> MSGVRAVRISIESACEKQVHEVGLDGTETYLPPLSMSQNLARLAQRIDFSQGSGSEEEEAAGTEGDAQEWPGAGSSADQDDEEGVVKFQPSLWPWDSVRNNLRSALTEMCVLYDVLSIVRDKKFMTLDPVSQDALPPKQNPQTLQLISKKKSLAGAAQILLKGAERLTKSVTENQENKLQRDFNSELLRLRQHWKLRKVGDKILGDLSYRSAGSLFPHHGTFEVIKNTDLDLDKKIPEDYCPLDVQIPSDLEGSAYIKVSIQKQAPDIGDLGTVNLFKRPLPKSKPGSPHWQTKLEAAQNVLLCKEIFAQLSREAVQIKSQVPHIVVKNQIISQPFPSLQLSISLCHSSNDKKSQKFATEKQCPEDHLYVLEHNLHLLIREFHKQTLSSIMMPHPASAPFGHKRMRLSGPQAFDKNEINSLQSSEGLLEKIIKQAKHIFLRSRAAATIDSLASRIEDPQIQAHWSNINDVYESSVKVLITSQGYEQICKSIQLQLNIGVEQIRVVHRDGRVIT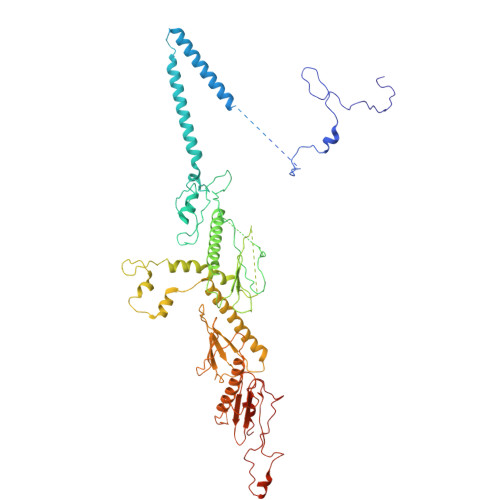LSYQEQELQDFLLSQMSQHQVHAVQQLAKVMGWQVLSFSNHVGLGPIESIGNASAITVASPSGDYAISVRNGPESGSKIMVQFPRNQCKDLPKSDVLQDNKWSHLRGPFKEVQWNKMEGRNFVYKMELLMSALSPCLL>MHIDNIENLSDREFDYIVVGGGSAGAAVAARLSEDPAVSVALVEAGPDDRGVPEVLQLDRWMELLESGYDWDYPIEPQENGNSFMRHARAKVMGGCSSHNACIAFWAPREDLDEWEAKYGATGWNAEAAWPLYKRLETNEDAGPDAPHHGDSGPVHLMNVPPKDPTGVALLDACEQAGIPRAKFNTGTTVVNGANFFQINRRADGTRSSSSVSYIHPIVEQENFTLLTGLRARQLVFDADRRCTGVDIVDSAFGHTHRLTARNEVVLSTGAIDTPKLLMLSGIGPAAHLAEHGIEVLVDSPGVGEHLQDHPEGVVQFEAKQPMVAESTQWWEIGIFTPTEDGLDRPDLMMHYGSV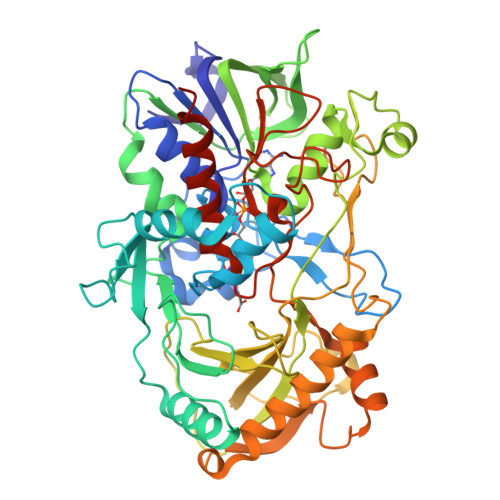PFDMNTLRHGYPTTENGFSLTPNVTHARSRGTVRLRSRDFRDKPMVDPRYFTDPEGHDMRVMVAGIRKAREIAAQPAMAEWTGRELSPGVEAQTDEELQDYIRKTHNTVYHPVGTVRMGAVEDEMSPLDPELRVKGVTGLRVADASVMPEHVTVNPNITVMMIGERCADLIRSARAGETTTADAELSAALA[8x]>[4x]GPGSAAHPPEIIRKPQNQGVRVGGVASFYCAARGDPPPSIVWRKNGKKVSGTQSRYTVLEQPGGISILRIEPVRAGRDDAPYECVAENGVG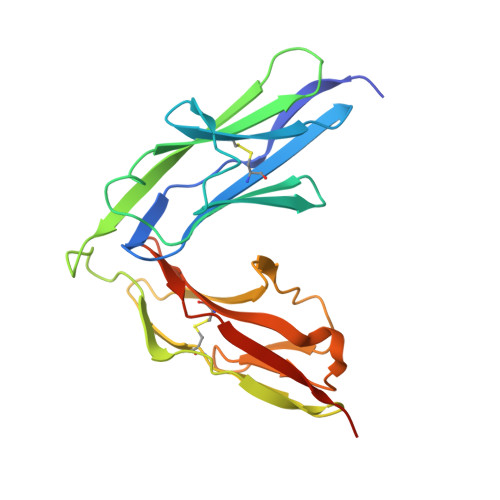DAVSADATLTIYEGDKTPAGFPVITQGPGTRVIEVGHTVLMTCKAIGNPTPNIYWIKNQTKVDMSNPRYSLKDGFLQIENSREEDQGKYECVAENSMGTEHSKATNLYVKVRRVPPTFS> MAIYADNSYSIGNTPLVRLKHFGHNGNVVVKIEGRNPSYSVKCRIGANMVWQAEKDGTLTKGKEIVEPTSGNTGIALAYVAAARGYKLTLTMPETMSLERKRLLCGLGVNLVLTEGAKGMKGAIAKAEEIVASDPSRYVMLKQFENPANPQIHRETTGPEIWKDTDGKVDVVVAGVGTGGSITGISRAIKLDFGKQITSVAVEPVESPVISQTLAGEEVKPGPHKIQGIGAGFIPKNLDLSIIDRVETVDSDTALATARRLMAEEGILAGISSGAAVAAADRLA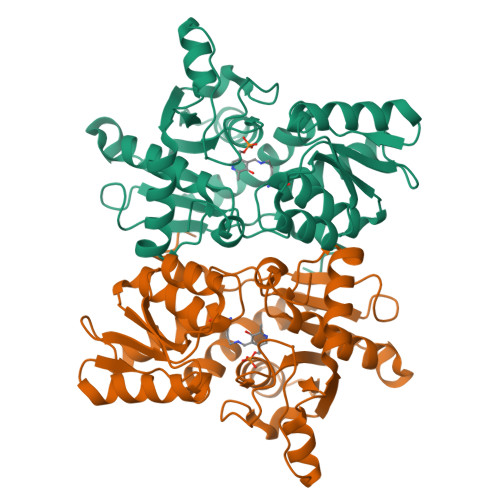KLPEFADKLIVVILPSASERYLSTALFEGIEG>[2x]SMDMPIMHDGDRYELVRDIGSGNFGVARLMRNRADGQLVAVKYIERGEKIDENVQREIINHRSLRHPNIIRFKEVILTPTHLAIVMEYASGGELFERICNAGRFSEDEARFFFQQLISGVSYCHSMQVCHRDLKLENTLLDGSTAPRLKICDFGYS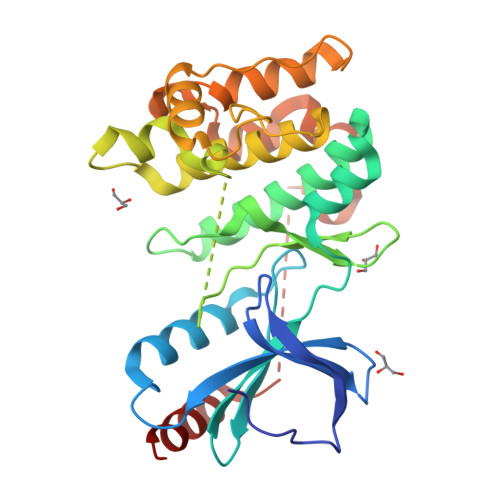KSSVLHSQPKSTVGTPAYIAPEVLLKKEYDGKVADVWSCGVTLYVMLVGAYPFEDPDEPKNFRKTIQRILGVQYSIPDYVHISPECQDLISRIFVANPATRITIPEIRNHPWFLKNLPADLMDDSTMSKQYEEPEQPMQSMDEIMQILAEATIP Formation of active HIV-1 reverse transcriptase (RT) proceeds via a structural maturation process that involves subdomain rearrangements and formation of an asymmetric p66/p66′ homodimer. The viral RNA codes for a p66 protein that forms an asymmetric homodimer in which the RNase H domain in one subunit becomes destabilized, leading to subsequent unfolding and proteolysis in order to form the active p66/p51 heterodimer. We utilized the isolated polymerase domain, p51, rather than p66, since the initial subdomain rearrangements are largely limited to this domain. Two different fingers/palm/connection (FPC) subdomain constructs containing the same interfaces that are present in the monomers and in the p51 subunit of the RT heterodimer were investigated using both NMR spectroscopy and X-ray crystallography.

The globular fingers, palm, and connection subdomains of FPC1 overlay well with those of both the p51 subunit of RT and the p51 monomer. Similar structural agreements were obtained using the FPC2 structure. Although crystal structures were obtained for both FPC1 and FPC2, the FPC constructs did not crystallize readily, perhaps due to the dynamic behavior of several loops.

> SDHHHHHHGPISPIETVPVKLKPGMDGPKVKQWPLTEEKIKALVEICTEMEKEGKISKIGPENPYNTPVFAIKKKDSTKWRKLVDFRELNKRTQDFWEVQLGIPHPAGLKKKKSVTVLDVGDAYFSVPLDEDFRKYTAFTIPSINNETPGIRYQYNVLPQGWKGSPAIFQSSMTKILEPFKKQNPDIVIYQYMDDLYVGSDLEIGQHRTKIEELRQHLLRWGLEPPFLWMGYELHPDKWTGSGSGGYDPSKDLIAEIQKQGQGQWTYQIYQEPSKNLKTGKYARKRGAHTNDVKQLTEAVQKITTESIVIWGKTPKFKLPIQKETWETWWTEYWQATWIPEWEFVN One key enzyme class is the poly-β-1,6-linked N-acetyl-d-glucosamine (PNAG)-degrading glycoside hydrolases, of which the canonical member is dispersin B (DspB) from CAZy family GH20. DispTs3, DispTs2 and DispLp all consist of a single domain with the expected (β/α)8 (TIM)-barrel fold for GH20 catalytic domains. The β-strands in the centre form a tunnel atop of which the active site is located in a groove, presumably to allow long chains of PNAG to bind. GH20 enzymes use a substrate-assisted catalytic mechanism, also referred to as neighbouring-group participation (NGP), in which the reaction proceeds via the formation and subsequent breakdown of a neutral oxazoline intermediate.

DispLp showed very low activity against both substrates, while DispTs2 showed the highest activity of the tested dispersins. In contrast, less than 1.3% of the sugars hydrolysed by DispTs2 and DspB were monosaccharides, indicating a preference for acting in an endo manner. 6-Ac-Cas has micromolar affinity towards DispTs2 and DispSf, with a Kd of 6 and 15 µM, respectively. In the active site of both enzymes 6-Ac-Cas was distorted into a 1S3 conformation, which is consistent with the proposed catalytic pathway of GH20 enzymes based upon the 1S3/4E (Michaelis complex/product) conformation for GH20 enzymes that was first observed for the S. marcescens chitobiase. The catalytic glutamate residues, Glu161 in DispTs2 and Glu156 in DispLp, are 3.4 and 3.6 Å away from the anomeric carbon of 6-Ac-Cas, respectively, consistent with closer positioning to the glycosidic oxygen during catalysis. Glu161 and Asp160 of DispTs2 are ∼5.2 Å apart, confirming that Glu161 is the general ‘glycosidic’ acid/base in catalysis. Arg13 of DispTs2 (and likewise Arg17 from DispLp) forms two hydrogen bonds to the C3 and C4 hydroxyls of 6-Ac-Cas with distances of approximately 2.8 Å. Glu300 of DispTs2 forms two hydrogen bonds to the C4 hydroxyl, at a distance of 2.7 Å, and to the C6 hydroxyl on the pyrrole ring, at a distance of 2.75 Å.

> QDQEKGITIDISRKHYTVETLKSLVDEISYNGGNYVQLHFSDNENYAIASEYLGQSSENTNNTYLTKNELLSLIAYSNDKDILVIPDIDLPAHSKGWLELIKKKDVKLYNDIVTDYSEETLDYYDNRVALDTVNQLLDEVLDLFYQPKFEGKQRIVLGGDEVSGSEVHQLDFIDFMNQIASTVKESKYEPQMWNDSITSEGIANLDDSFSILYWQQSTLSSGEESLNVEDFENWGFSVYNYNAYSLYFLPSNGFTQEDINEQMDYMNWAYAHNKFFYISDYYHAVETSNVKGSSLTFWGEHATDLSQKKLLKQELPLIRHYLNL PCNA is a ring-shaped homotrimeric protein, with each subunit consisting of two domains connected by a flexible linker called the inter-domain connecting loop (IDCL). CAF-1 association with replicating DNA, and the targeting of newly synthesized histones to sites of DNA replication and repair requires its interaction with proliferating cell nuclear antigen (PCNA), the eukaryotic sliding clamp that acts as a processivity factor for polymerases during DNA synthesis. Recruitment of PCNA-interacting proteins to replication forks is generally mediated by a conserved sequence in these proteins called a PCNA-interacting protein (PIP) motif that interacts with PCNA in a region between the two domains on a single subunit near the IDCL. In this study, we focused on three separation-of-function amino acid substitutions in PCNA that cause defective gene silencing and exhibit reduced CAF-1 association with chromatin in vivo, as well as inhibit binding to CAF-1 in vitro partially or completely (D41A/D42A, R61A/D63A, and L126A/I128A).

The X-ray crystal structure of the D41A/D42A mutant protein was determined to a resolution of 3.05 Å. The D41A/D42A substituitions are located on the front face of PCNA in loop D (residues 41–44) between β strands C1 and D1. The D41A/D42A substitutions are located on the front of the PCNA ring in loop D (residues 41 to 44), which is approximately 10 Å away from the canonical PIP-interacting region. The global structure of the mutant PCNA trimer is very similar to the structure of the wild-type PCNA trimer. Compared to the wild-type structure, there are significant backbone changes in the structure of the D41A/D42A mutant PCNA protein in loop D. The α carbon of residue 42 has moved by 1.2 Å relative to its position in the wild-type PCNA structure, and the α carbon of residue 43 has moved by 1.0 Å. These backbone changes in loop D and the substitutions of the shorter alanine sidechains at residues 41 and 42 are the only significant changes in the structure of the mutant PCNA protein compared to the structure of the wild-type PCNA protein. One of the three PCNA mutations, D41A/D42A, is located directly within one of the loops that defines this cavity. In the structure of the D41A/D42A mutant PCNA protein, the replacement of the larger, negatively charged aspartate residues with smaller, non-polar alanine residues causes alterations (>1 Å) in the positions of the backbone of several amino acid side chains that line the edges of the surface cavity, including residues 41 and 43 in loop D and residue 123 in the IDCL. Together, these changes result in the formation of a smaller, more “closed” surface cavity compared to the cavity in the wild-type structure.

> MHHHHHHMLEAKFEEASLFKRIIDGFKDCVQLVNFQCKEDGIIAQAVAASRVLLVSLEIGVEAFQEYRCDHPVTLGMDLTSLSKILRCGNNTDTLTLIADNTPDSIILLFEDTKKDRIAEYSLKLMDIDADFLKIEELQYDSTLSLPSSEFSKIVRDLSQLSDSINIMITKETIKFVADGDIGSGSVIIKPFVDMEHPETSIKLEMDQPVDLTFGAKYLLDIIKGSSLSDRVGIRLSSEAPALFQFDLKSGFLQFFLAPKFNDEE Phenotype switching in Bacillus subtilis requires an all-or-none promoter binding of multiple ComK proteins. ComK target promoters consist of two elements (hereafter) separated by spacer sequences of variable length. Each box in a promoter contains an adenine–thymine (AT)-rich sequence. Cryo-EM structures of the complex between ComK and its promoter demonstrate that this coupling is due to mechanical forces that alter DNA curvature.

We determined 2D class averages of ComK bound to promoters with spacers of 8 bp (addAB: 57 bp, 35.2 kDa), 18 bp (comG: 93 bp, 57.5 kDa), and 31 bp (comK: 93 bp, 57.5 kDa). Three observations are notable: (i) the extra density bound to DNA is confined to two locations that agree with the position of box 1 and box 2, thus assigning this density to ComK; (ii) the DNA in these complexes is not looped, and (iii) only a few particles with ComK density on only one box are found for promoters with 8 and 31 bp spacers. To determine the precise arrangement of ComK on the DNA, we reconstructed the 3D maps of the complexes with spacers of 8 and 18 bp. The 3D maps show that ComK molecules in the two boxes face the same side of the DNA. In addition, we find a pseudo C2-symmetry of the protein density in each box, indicating two molecules of ComK per box, i.e., four per promoter, in excellent accord with the Hill exponents and a previous report. Indeed, a fit of our 3D density with an atomistic representation of the addAB promoter (8 bp spacer) that agrees well with our smFRET values, suggests that ComK faces the minor groove by forming contacts with the thymine bases of the A-tracts. Widening the minor groove by ComK would lower DNA curvature around a box, thus affecting the width of the minor groove at the second box. For instance, boxes in the natural promoters addAB and comG are one and two helical turns away from each other, respectively, thus leading to symmetric arrangements in which ComK always faces the same side of the DNA. Similarly, the coupling free energy (−ΔgJ) drops from 5.8 ± 0.9 kBT (8 bp) over 4.5 ± 1.2 kBT (18 bp) to 1.9 ± 0.1 kBT (31 bp). The result shows that spacer length is key for allostery, in line with the idea that reducing promoter curvature is the main origin for allosteric signal transmission.

> GGAGAGATGTGCGGAGATAATCAGCTTTTTATATGTGAAAAGGCCGTTTTTACCAATAGATCAGATTGGTCATTTTCG;> CGAAAATGACCAATCTGATCTATTGGTAAAAACGGCCTTTTCACATATAAAAAGCTGATTATCTCCGCACATCTCTCC>[2x]MAAAAVVAATVPAQSMGADGASSVHWFRKGLRLHDNPALLAAVRGARCVRCVYILDPWFAASSSVGINRWRFLLQSLEDLDTSLRKLNSRLFVVRGQPADVFPRLFKEWGVTRLTFEYDSEPFG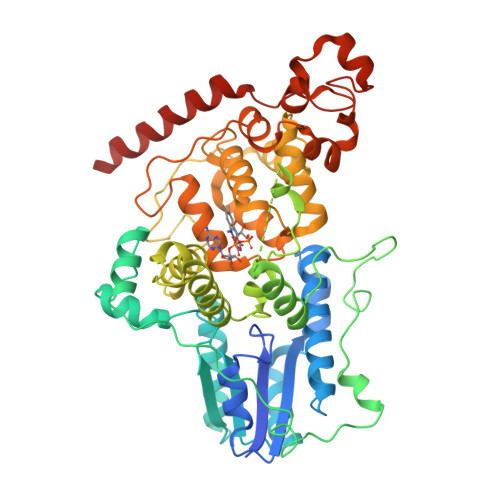KERDAAIMKMAKEAGVEVVTENSHTLYDLDRIIELNGQKPPLTYKRFQALISRMELPKKPAVAVSSQQMESCRAEIQENHDDTYGVPSLEELGFPTEGLGPAVWQGGETEALARLDKHLERKAWVANYERPRMNANSLLASPTGLSPYLRFGCLSCRLFYYRLWDLYKKVKRNSTPPLSLFGQLLWREFFYTAATNNPRFDRMEGNPICIQIPWDRNPEALAKWAEGKTGFPWIDAIMTQLRQEGWIHHLARHAVACFLTRGDLWVSWESGVRVFDELLLDADFSVNAGSWMWLSCSAFFQQFFHCYCPVGFGRRTDPSGDYIRRYLPKLKGFPSRYIYEPWNAPESVQKAAKCIIGVDYPRPIVNHAETSRLNIERMKQIYQQLSRY>MAESQALSD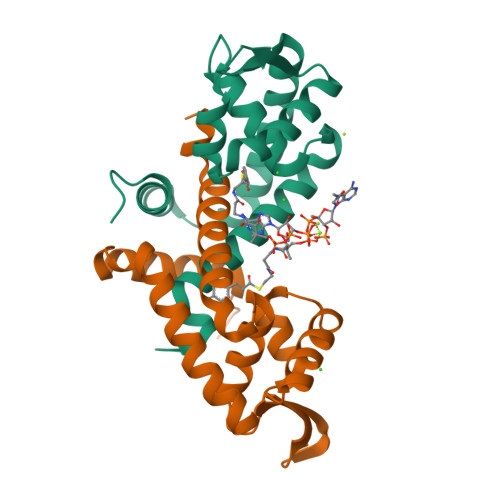DIGFLLSRVGGMVLGAVNKALVPTGLRVRSYSVLVLACEQAEGVNQRGVAATMGLDPSQIVGLVDELEERGLVVRTLDPSDRRNKLIAATEEGRRLRDDAKARVDAAHGRYFEGIPDTVVNQMRDTLQSIAFPTFVE[2x]At the inner surface of fly photoreceptor rhabdomeric membranes, the master scaffold protein INAD (encoded by inaD for inactivation no after potential D and contains 5 PDZ domains arranged in tandem) forms stoichiometric multi-molecular complexes with phospholipase Cβ (NORPA), Ca2+-permeable transient receptor potential (TRP) channel and eye-specific protein kinase C (eye-PKC). In this study, we show that the PDZ45 tandem of INAD functions as a supramodule binding to the entire C-terminal coiled-coil domain and PDZ-binding motif of NORPA (CC-PBM) with an unexpectedly high affinity. Our biochemical and structural studies demonstrate that INADL PDZ89 forms a supramodule and binds to the entire C-terminal coiled-coil domain of PLCβ4 in a manner that is strikingly similar to that of the INAD–NORPA complex. The striking similarity between the PDZ scaffold and PLCβ interactions at the molecular level might point to an evolutionarily conserved molecular adaption in PLCβ signaling in the animal kingdom.

To elucidate the molecular mechanism governing the interaction between PLCβ4 and INADL, we determined the crystal structure of the INADL PDZ89–PLCβ4 CC-PBM complex. To facilitate the complex crystal growth, we also substituted the eight Lys residues in the α2 helix of PLCβ4 CC with Ala. Furthermore, we discovered that covalently linking INADL PDZ89 with the PLCβ4 CC8KA-PBM was necessary to obtain diffraction-quality crystals of the complex. The complex structure was determined by the single-wavelength anomalous dispersion method using gold derivatives at a resolution of 2.8 Å. Strikingly, the overall architecture of the PLCβ4 CC8KA-PBM–INADL PDZ89 complex is remarkably similar to that of the NORPA–INAD complex. In the complex, PDZ89 forms an integral structural unit and extensively binds to the CC-PBM domain of PLCβ4, burying a total of ~1211 Å2 surface area. In the complex, the formation of a supramodule between PDZ8 and PDZ9 is mediated by a number of hydrophobic residues from both domains. Like that of the INAD–NORPA complex, the binding interface of the INADL PDZ89–PLCβ4 CC-PBM complex can be divided into three distinct sites: the PDZ9–PBM interaction site (site 1), the PDZ9/CC interaction site (site 2), and the PDZ8–CC binding site (site 3). In site 1, the last four amino acids (ATVV) of the PLCβ4 PBM bind to the canonical αB/βB-pocket of PDZ9. In site 3, the carboxyl group of E1164 from α4 of the PLCβ4 CC forms hydrogen bonds with the backbone of the GLGL loop of PDZ8 by mimicking the classical carboxyl group–GLGF binding found in all PDZ–target interactions.

> EGELIPQVRIEDLKQMAAYLAHLAAQQAELNSLKAAHAAEHSTMQKLHCTQVDKIVAQYDKEKSTHEKILEKAMKKKGGSNCLEIKKETEIKIQTLTTDHKSKVKEIVAQHTKEWSEMINTHSAEEQEIRDLHLSQQCELLRKLLINAHEQQTQQLKLSHDRESKEMRAHQAKISMENSKAISQDKSIKNKAERERRVRELNSSNTKKFLEERKRLAMKQSKEMDQLKKVQLEHLEFLEKQNEQAKEMQQMVKLEAEMDRRPATVV;> LSVDPATCPIVPGQEMIIEISKGRSGLGLSIVGGKDTPLNAIVIHEVYEEGAAARDGRLWAGDQILEVNGVDLRNSSHEEAITALRQTPQKVRLVVYRDEAHYRDEENLEIFPVDLQKKAGRGLGLSIVGKRNGSGVFISDIVKGGAADLDGRLIQGDQILSVNGEDMRNASQETVATILKCAQGLVQLEIGRLRAGSWTSARTTGGGSGGGGSGG> DANLLNDRVLRAMLKAEETCAPSVSYFKCVQKEVLPSMRKIVATWMLEVCEEQKCEEEVFPLAMNYLDRFLSLEPVKKSRLQLLGATCMFVASKMKETIPLTAEKLCIYTDNSIRPEELLQMELLLVNKLKWNLAAMTPHDFIEHFLSKMPEAEENKQIIRKHAQTFVALCATDVKFISNPPSMVAAGSVVAAVQGLNLRSPNNFLSYYRLTRFLSRVIKCDPDCLRACQEQIEALLESSLRQAQQNMD;> GEFATSRYEPVAEIGVGAYGTVYKARDPHSGHFVALKSVRVPNGEEGLPISTVREVALLRRLEAFEHPNVVRLMDVCATSRTDREIKVTLVFEHVDQDLRTYLDKAPPPGLPAETIKDLMRQFLRGLDFLHANCIVHRDLKPENILVTSGGTVKLADFGLARIYSYQMALTPVVVTLWYRAPEVLLQSTYATPVDMWSVGCIFAEMFRRKPLFCGNSEADQLGKIFDLIGLPPEDDWPRDVSLPRGA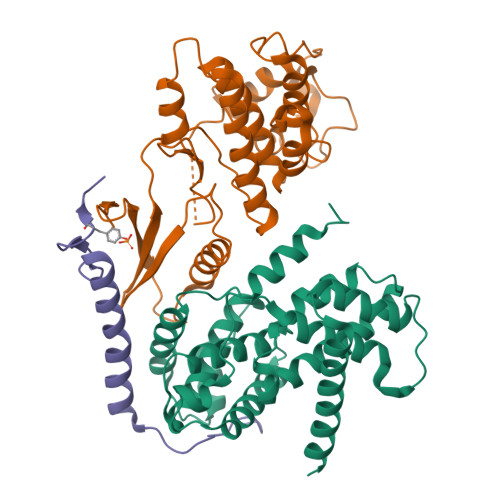FPPRGPRPVQSVVPEMEESGAQLLLEMLTFNPHKRISAFRALQHSYLHKDEGNPE;> GEFKPSACRNLFGPVDHEELTRDLEKHCRDMEEASQRKWNFDFQNHKPLEGKYEWQEVEKGSLPEFYYRPPKGACKVPAQES>GMQENTRLRIAIQKSGRLSKESIELLSECGVKMHIHEQSLIAFSTNLPIDILRVRDDDIPGLIFDGVVDLGIIGENVLEENELERQSLGENPSYKLLKKLDFGYCRLSLALPQENKFQNLKDFEGLRIATSYPQLLKRFMKENGINYKNCTLTGSVEVAPRANLADAICDLVSSGATLQANNLKEVKVIYESRACLIQKENALSKEKQ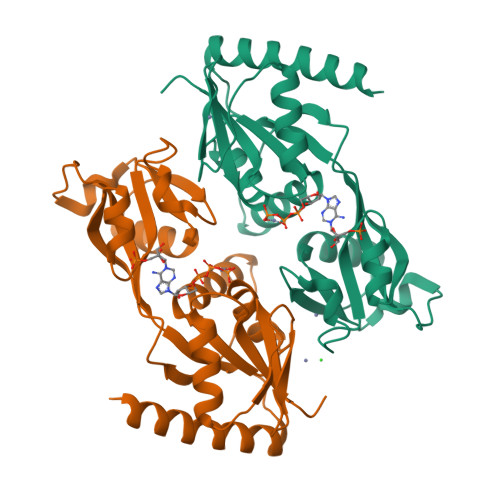ALVDKIMLRVAGVMQARE[2x]> GPVCAEASDVYSPCMIASTPPAPFSDVTAVTFDLINGKITPVGDDNWNTHIYNPPIMNVLRTA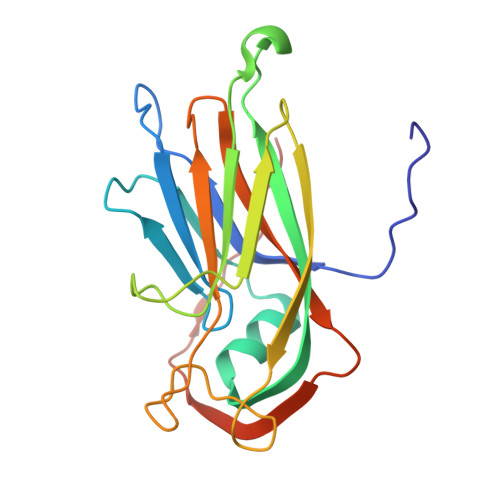AWKSGTIHVQLNVRGAGVKRADWDGQVFVYLRQSMNPESYDARTFVISQPGSAMLNFSFDIIGPNSGFEFAESPWANQTTWYLECVATNPRQIQQFEVNMRFDPNFRVAGNILMPPFPLSTETPPL>[2x]HHHHHHFNLPPGNYKKPKLLYCSNGGHFLRILPDGTVDGTRDRSDQHIQLQLSAESVGEVYIKSTE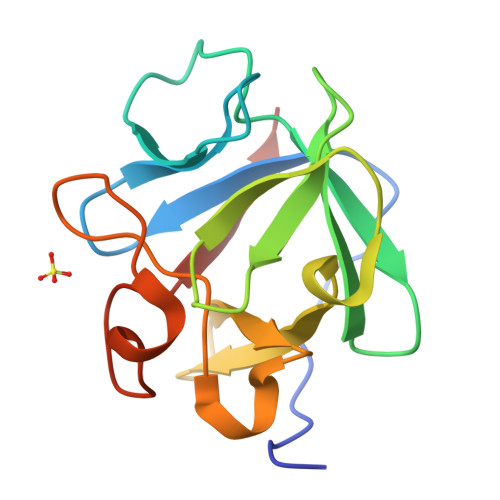TGQYLAMDTDGLLYGSQTPNEECLFLERLEENHYNTYISKKHAEKNWFVGLKKNGSTKRGPRTHYGQKAILFLPLPVSSD>MSHHHHHHSMDMSAWRLLLTRPAEESAALARVLADAGIFSSSLPLLETEPLPLTPAQRSIIFELLNYSAVIVVSKPAARLAIELIDEVWPQPPMQPWFSVGSATGQ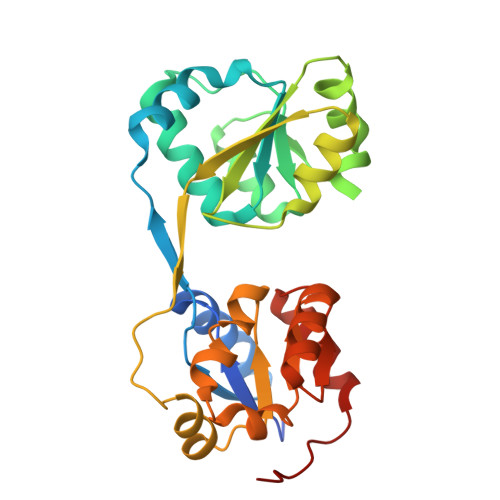ILLDYGLDASWPEQGDDSEALLDHPRLKQAIAVPGSRVLIMRGNEGRELLAEQLRERGVGVDYLPLYRRYLPQHAPGTLLQRVEVERLNGLVVSSGQGFEHLLQLAGDSWPDLAGLPLFVPSPRVASLAQAAGARNVIDCRGASAAALLAALRDQPQPAVKAY[2x]>GSHMAKTVILDHDGNKDDFVAMILLLSNPKKVNLIGCICTDADCFVENGFDVTGKIMCAMHRLIKTPLFPIGKSTATAVNAFPTEWRFSAKNLDDMPFLNIVEDVALWEKLKPENEAHNGQQLLADLVMKSKEKVTVCVTGPLSNMAWCIEKYGEAFTSKVEECVIMGGAVDVGGNVFLPTTDGSAEWNIYWDPPAAKKVLCCPNIRCVLFSLDATNTVPVRSVDVKGFGAQNQYLLSQMVGTM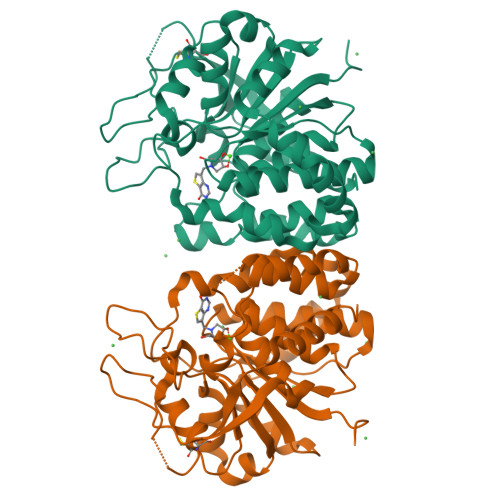WAMSTHEEILRDGDAYYAWDALTAAYILEPTIATLEPVALDVDVSKGKSEGRTPRASGEGKPCVHVARNPSKQMFHDLVFASTRVC[4x]>[4x]GSHMSNPFEEYDGGHVVLTDALGRHSLWPAGIAVPAGWSVRHGTDSREGCLAHIEHHWTDLRPTGPAVERAPAGACVHELFEAQAARAPDAVALLHEADELTYGALNERANRLAHRLVGLGVAPGTLVGVHLERGFDMVVALLAVLKAGGGYTMLDPQFPVERLALSLEDTGAPLLVTSRPLSGRLTGTTTLYVEDEAASDAPAGN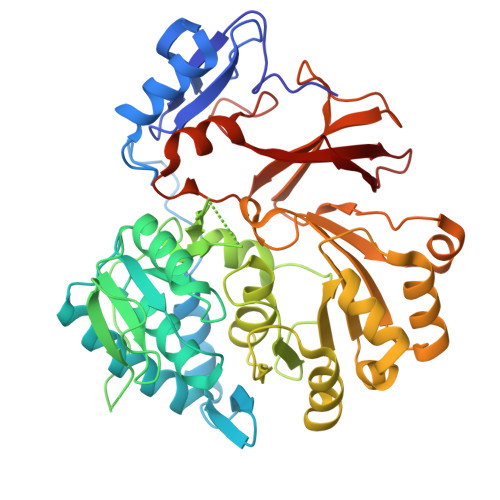LATGVGPEDVACVMFTSGSTGRPKGVMSPHRALTGTYLGQDYAGFGPDEVFLQCSPVSWDAFGLELFGALLFGARCVLQSGQNPDPLEIGELVARHGVTMLQLSASLFNFLVDEVPEAFEGVRYAITGGEPASVPHVAKARRDHPALRLGNGYGPAESMGFTTHHAVVAGDLSGTALPIGVPLAGKRAYVLDDDLKPAANGALGELYVAGAGLAHGYVSRPALTAERFVADPFAGPGGERMYRTGDLARRRADGVLEYVGRAD>[2x]MKKIIYIATIGITLLTTSCDDFLDRQVPQGIVTGDQIASPEYVDNLVISAYAIWATGDDINSSFSLWNYDVRSDDCYKGGSGTEDGGVFNALEISKGINTTDWNINDIWKRLYQCITRANTALQSLDQMDEKTYPLKNQRIAEMRFLRGHAHFMLKQLFKKIVIVNDENMEPDAYNELSNTTYTNDEQWQKIADDFQFAYDNLPEVQIEKGRPAQAAAAAYLAKTYLYKAYRQDGADNALTGINEEDLKQVVKYTDPLIMAKGGYGLETDYSMNFLPQYENGAESVWAIQYSINDGTYNGNLNWGMGLTTPQILGCCDFHKPSQNLVNAFKTDSQGKPLFSTYDNENYEVATDNVDPRLFHTVGMPGFPYKYNEGYIIQKNDDWSR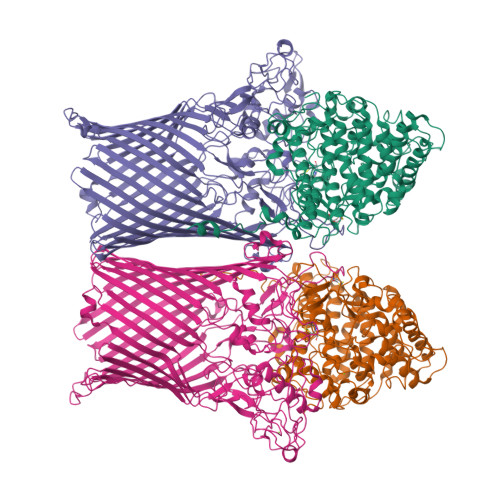SKGLYGYYVSLKENVDPDCDCLKKGSYWASSLNHIVIRYADVLLMRAEALIQLNDGRITDAISLINEVRSRAAGSTMLIFNYKEDYGVNFKVTPYDLKAYAQDEAMKMLKWERRVEFGMESSRFFDLVRWGEAKDVINAYYVTEASRCSIYKNAGFTENKNEYLPVPFEQISASNGNYTQNFGWHHHHHH;>[2x]MPGIMKNKKLLCSVCFLFAFMSALWGQNITVKGNVTSKTDGQPIIGASVVETTATTNGTITDFDGNFTLSVPVNSTLKITYIGYKPVTVKAAAIVNVLLEEDTQMVDEVVVTGYTTQRKADLTGAVSVVKVDEIQKQGENNPVKALQGRVPGMNITADGNPSGSATVRIRGIGTLNNNDPLYIIDGVPTKAGMHELNGNDIESIQVLKDAASASIYGSRAANGVIIITTKQGKKGQIKINFDASVSASMYQSKMNVLNTEQYGRAMWQAYVNDGENPNGNALGYAYNWGYNADGNPVLYGMTLSKYLDSKNTMPVADTDWFDEITRTGVIQQYNLSVSNGSEKGSSFFSLGYYKNLGVIKDTDFDRFSARMNSDYKLIDDILTIGQHFTLNRTSEVQAPGGIIETALDIPSAIPVYASDGSWGGPVGGWPDRRNPRAVLEYNKDNRYTYWRMFGDAYVNLTPFKGFNLRSTFGLDYANKQARYFTYPYQEGTQTNNGKSAVEAKQEHWTKWMWNAIATYQLEVGKHRGDVMIGMELNREDDSHFSGYKEDFSILTPDYMWPDAGSGTAQAYGAGEGYSLVSFFGKMNYSYADRYLLSLTLRRDGSSRFGKNHRYATFPSVSLGWRITQENFMKELTWLDDLKLRASWGQTGNQEISNLARYTIYAPNYGTTDSFGGQSYGTAYDITGSNGGGVLPSGFKRNQIGNDNIKWETTTQTNVGIDFSLFKQSLYGSLEYYYKKATDILTEMAGVGVLGEGGSRWINSGAMKNQGFEFNLGYRNKTAFGLTYDLNGNISTYRNEILELPETVAANGKFGGNGVKSVVGHTYGAQVGYIADGIFKSQDEVDNHATQEGAAVGRIRYRDIDHNGVIDERDQNWIYDPTPSFSYGLNIYLEYKNFDLTMFWQGVQGVDIISDVKKKSDFWSASNVGFLNKGTRLLNAWSPTNPNSDIPALTRSDTNNEQRVSTYFVENGSFLKLRNIQLGYTVPAVISKKMRMDRLRFYCSAQNLLTIKSKNFTGEDPENPNFSYPIPVNITFGLNIGF4-(1H-imidazol-1-yl)benzoic 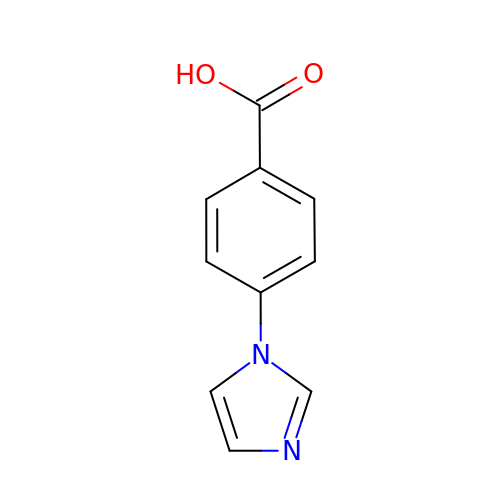acid | C10 H8 N2 O2 | LFIDZIWWYNTQOQ-UHFFFAOYSA-N> MFELVDNIAQTAVIKVIGVGGGGGNAVNHMAKNNVEGVEFICANTDAQALKNIAARTVLQLGPGVTKGLGAGANPEVGRQAALEDRERISEVLEGADMVFITTGMGGGTGTGAAPIIAEVAKEMGILTVAVVTRPFPFEGRKRMQIADEGIRALA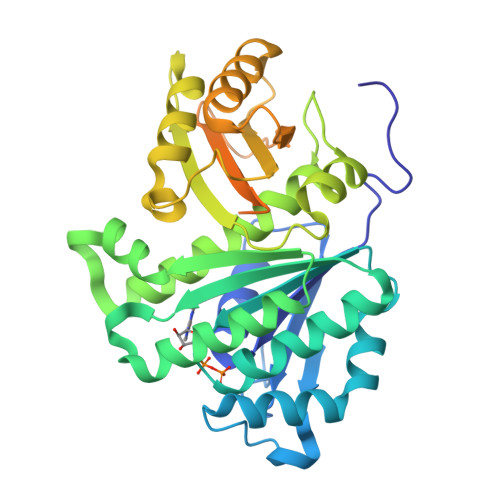ESVDSLITIPNEKLLTILGKDASLLAAFAKADDVLAGAVRGISDIIKRPGMINVDFADVKTVMSEMGMAMMGTGCASGPNRAREATEAAIRNPLLEDVNLQGARGILVNITAGPDLSLGEYSDVGNIIEQFASEHATVKVGTVIDADMRDELHVTVVATGLGARLEKPVKVVDNTVQGSAAQAAAPAQREQQSVNYRDLDRPTVMRNQSHGSAATAAKLNPQDDLDYLDIPAFLRRQAD>[3x]MGSSHHHHHHSAALEVLFQGPDYKFWYTQPVPKINDEFNESVNEPFISDNKVEDVRKDEYKLPPGY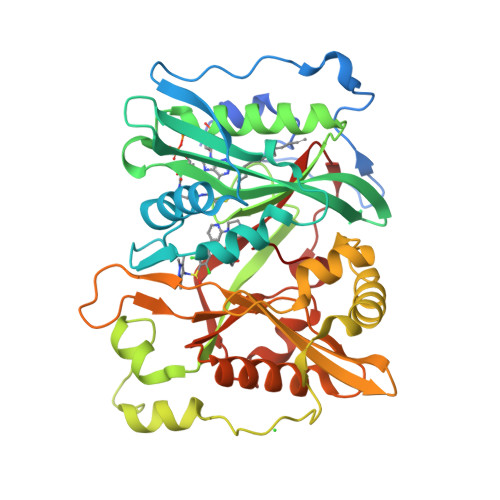SWYVCDVKDEKDRSEIYTLLTDNYVEDDDNIFRFNYSAEFLLWALTSPNYLKTWHIGVKYDASNKLIGFISAIPTDICIHKRTIKMAEVNFLCVHKTLRSKRLAPVLIKEITRRINLENIWQAIYTAGVYLPKPVSDARYYHRSINVKKLIEIGFSSLNSRLTMSRAIKLYRVEDTLNIKNMRLMKKKDVEGVHKLLGSYLEQFNLYAVFTKEEIAHWFLPIENVIYTYVNEENGKIKDMISFYSLPSQILGNDKYSTLNAAYSFYNVTTTATFKQLMQDAILLAKRNNFDVFNALEVMQNKSVFEDLKFGEGDESLKYYLYNWKCASFAPAHVGIVLL1-[6-(6-methoxyisoquinolin-7-yl)-1,3-benzothiazol-2-yl]-3-(2-oxidanylideneethyl)urea | C20 H16 N4 O3 S | 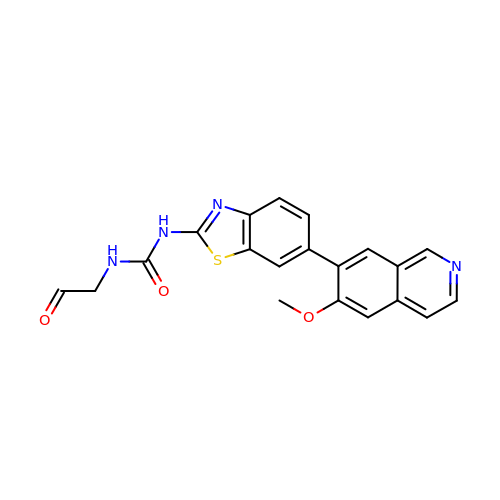BTOGRSOLMDUWDV-UHFFFAOYSA-N> SSQSQSPTED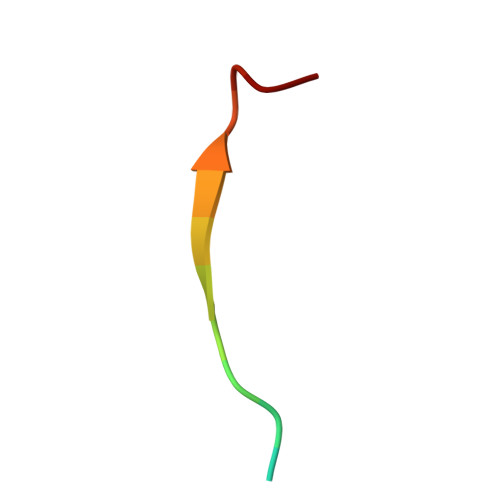DENES> MGANDYVPSPITINTSTLPVVVIGPADAHTYP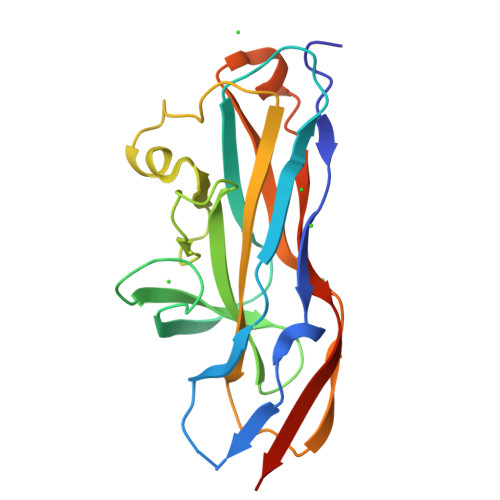RVIGELTGTSNQYIFNGGSLIALMRGKFTPTLPKIGKITYNFRQGNNTQSSDFDIFDTGVPGLGIIIGMAGYWPATPLVPINSSSIYIDPVAANTNPNAYNGATGSFGARLYVAFVATGRLPNGYVTIPTKQLGHILLESNRASLNNKRLTAPVMLNGGRIQVQSLEHHHHHH>[2x]MHHHHHHSSGRENLYFQGHMDRLITLVVSYSIAFSIFALATMAVVYGKWLYYFEIDFLNIPDLADMTKDEIKRNYDVLITYLSPFYDGALHLPTLDMSTNGRIHFVDVKNILVKIQYVMYATIMIAVIGGIYLLKKKNEKFLLHGSILTIIFPIALMLPIAINFEKSFVLFHKLLFSNDYWVFDPEKDPIILMLPEEFFMHAACAILLFILGGSILCYSLYRYLVKKKRMSQKKFSA

Here, we report the crystal structure of the Lit enzyme from Bacillus cereus and describe its mechanism of action. Lit consists of four transmembrane helices with an extracellular cap. Conserved residues map to the cap-membrane interface. They include two catalytic histidines that function to effect unimolecular transacylation. The reaction involves acyl transfer from the sn-2 position of the glyceryl moiety to the amino group on the N-terminal cysteine of the substrate via an 8-membered ring intermediate.

A hexahistidine N-terminally tagged variant of Lit from B. cereus was over-expressed in E. coli and was crystallised by the in meso method with monoolein as the host lipid. Two structures were solved; one at 2.27 Å, the other at 1.95 Å. The former, in space group P21, displayed type I crystal packing. Root mean-square deviations calculated for Cα atoms in the different structures (211 to 216 residues) range from 0.21 to 0.40 Å. Monoolein molecules from the mesophase in which crystallogenesis occurs coat the protein surface recapitulating the native membrane and occupy a volume inside the protein. Notably, two structured monoolein molecules that derive from the crystallisation process reside with their glyceryl head groups coordinated with the two conserved histidines. These lipids are considered surrogates of the DAG moiety of the DA-BLP substrate and serve to reinforce the view that they sit proximal to the active site of Lit.Cross reacting material (CRM197) is widely used as a carrier protein in conjugate vaccines. CRM197 protein is a nontoxic variant of diphtheria toxin (DT, molecular weight: ~58 kDa) with a single mutation (Glycine to Glutamate substitution at position 52) that eliminates its toxicity. CRM197 is synthesized as a single chain holoprotein, which comprises two domains fragment A (catalytic domain) and fragment B (transmembrane domain), bound together by a disulfide bridge. The B domain contains a subdomain for binding to the HB-EGF cell receptor and another subdomain for translocation into eukaryotic cells.

To verify if the rCRM197 produced from insoluble inclusion body protein have the overall similar 3D structure of the protein, we determined the X-ray crystal structure of rCRM197. The asymmetric unit contains four molecules of rCRM197 (chains A, B, C and D). The four chains interact as dimers (chains A–B and chains C–D) by domain swapping, with each monomer in ‘open’ conformation, a typical packing that has already been described for both DT and CRM197. The overall fold of the monomer rCRM197 is equivalent to C7-CRM197, with an overall RMSD of 0.34 Å for 451 out of 498 superimposed Cα atoms. The dimers in the crystal structure of rCRM197 and C7-CRM197, are equivalent. Furthermore, previous studies showed that the substitution G52E induces the dislocation of the active-site loop CL2 in C7-CRM197 with respect to DT. In our crystal structure of rCRM197, we have also observed a low electron density in the active loop CL2, consistent with the previous results. This confirms the structural basis of lack of toxicity in rCRM197. The structure revealed that the disulfide bond is conserved in rCRM197. In conclusion, rCRM197 conserves the overall folding, making it structurally equivalent to C7-CRM197, which is used in many licenced conjugate vaccine such as meningitis, pneumococcal conjugate vaccine etc..

>[4x]GADDVVDSSKSFVMENFSSYHGTKPGYVDSIQKGIQKPKSGTQGNYDDDWKEFYSTDNKYDAAGYSVDNENPLSGKAGGVVKVTYPGLTKVLALKVDNAETIKKELGLSLTEPLMEQVGTEEFIKRFGDGASRVVLSLPFAEGSSSVEYINNWEQAKALSVELEINFETRGKRGQDAMYEYMAQACAGNRVRRSVGSSLSCINLDWDVIRDKTKTKIESLKEHGPIKNKMSESPNKTVSEEKAKQYLEEFHQTALEHPELSELKTVTGTNPVFAGANYAAWAVNVAQVIDSETADNLEKTTAALSILPGIGSVMGIADGAVHHNTEEIVAQSIALSSLMVAQAIPLVGELVDIGFAAYNFVESIINLFQVVHNSYNRPAYSPGHKTQPFLHDGYAVSWNTVEDSIIRTGFQGESGHDIKITAENTPLPIAGVLLPTIPGKLDVNKSKTHISVNGRKIRMRCRAIDGDVTFCRPKSPVYVGNGVHANLHVAFHRSSSEKIHSNEISSDSIGVLGYQKTVDHTKVNSKLSLFFEIKS>MSLQESSLVLSNGLGFVDTPYKAGTLEVDDTEDLIINCDEVDCTTFVEYALAMALCPQQGDEMQEGDFARNLQRIRYRDGKIDGYTSRLHYISDWINNAVRQGLLEDVTAAYSPFKQKLSLSYMSTHPELYKSLKNSPENVAQMAKYEKALSGKEVHYLPKDKLEPDGLPWIKNGDIIA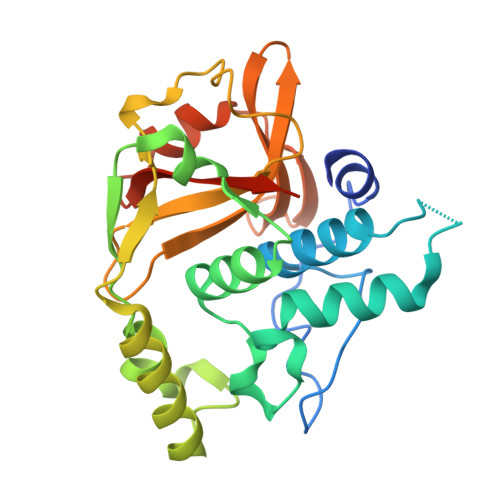LTTNTPGLDVSHMGIAIYIKGQLHLLHASSKEGKVVVGKTALSQMLKDRKSLTGIRVLRMKKEGHHHHHH[2x]> GSILTRWLLIPPVNARLIGRYRDYRRHGASAFSATLGCFWMILAWIFIPLEHPRWQRIRAEHKNLYPHINASRPRPLDPVRYLIQTCWLLIGASRKETPKPRRRAFSGLQNIRGRYHQWMNELPERVSHKTQHLDEKKELGHLSAGARRLILGIIVTFSLILALICVTQPFNPLAQFIFLMLLWGVALIVRRMPGRFSALMLIVLSLTVSCRYIWWRYTSTLNWDDPVSLVCGLILLFAETYAWIVLVLGYFQVVWPLNRQPVPLPKDMSLWPSVDIFVPTYNEDLNVVKNTIYASLGIDWPKDKLNIWILDDGGREEFRQFAQNVGVKYIARTTHEHAKAGNINNALKYAKGEFVSIFDCDHVPTRSFLQMTMGWFLKEKQLAMMQTPHHFFSPDPFERNLGRFRKTPNEGTLFYGLVQDGNDMWDATFFCGSCAVIRRKPLDEIGGIAVETVTEDAHTSLRLHRRGYTSAYMRIPQAAGLATESLSAHIGQRIRWARGMVQIFRLDNPLTGKGLKFAQRLCYVNAMFHFLSGIPRLIFLTAPLAFLLLHAYIIYAPALMIALFVLPHMIHASLTNSKIQGKYRHSFWSEIYETVLAWYIAPPTLVALINPHKGKFNVTAKGGLVEEEYVDWVISRPYIFLVLLNLVGVAVGIWRYFYGPPTEMLTVVVSMVWVFYNLIVLGGAVAVSVESKQVRRSHRVEMTMPAAIAREDGHLFSCTVQDFSDGGLGIKINGQAQILEGQKVNLLLKRGQQEYVFPTQVARVMGNEVGLKLMPLTTQ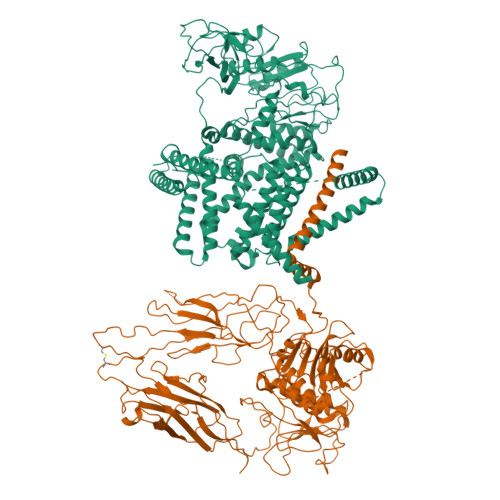QHIDFVQCTFARADTWALWQDSYPEDKPLESLLDILKLGFRGYRHLAEFAPSSVKGIFRVLTSLVSWVVSFIPPRPERSETAQPSDQALAQQHHHHHHLEHHHHHH;> MKRKLFWICAVAMGMSAFPSFMTQATPATQPLINAEPAVAAQTEQNPQVGQVMPGVQGADAPVVAQNGPSRDVKLTFAQIAPPPGSMVLRGINPNGSIEFGMRSDEVVTKAMLNLEYTPSPSLLPVQSQLKVYLNDELMGVLPVTKEQLGKKTLAQMPINPLFISDFNRVRLEFVGHYQDVCEKPASTTLWLDVGRSSGLDLTYQTLNVKNDLSHFPVPFFDPSDNRTNTLPMVFAGAPDVGLQQASAIVASWFGSRSGWRGQNFPVLYNQLPDRNAIVFATNDKRPDFLRDHPAVKAPVIEMINHPQNPYVKLLVVFGRDDKDLLQAAKGIAQGNILFRGESVVVNEVKPLLPRKPYDAPNWVRTDRPVTFGELKTYEEQLQSSGLEPAAINVSLNLPPDLYLMRSTGIDMDINYRYTMPPVKDSSRMDISLNNQFLQSFNLSSKQEANRLLLRIPVLQGLLDGKTDVSIPALKLGATNQLRFDFEYMNPMPGGSVDNCITFQPVQNHVVIGDDSTIDFSKYYHFIPMPDLRAFANAGFPFSRMADLSQTITVMPKAPNEAQMETLLNTVGFIGAQTGFPAINLTVTDDGSTIQGKDADIMIIGGIPDKLKDDKQIDLLVQATESWVKTPMRQTPFPGIVPDESDRAAETRSTLTSSGAMAAVIGFQSPYNDQRSVIALLADSPRGYEMLNDAVNDSGKRATMFGSVAVIRESGINSLRVGDVYYVGHLPWFERVWYALANHPILLAVLAAISVILLAWVLWRLLRIISRRRLNPDNE> QHGKKDSKITDHFMRLPK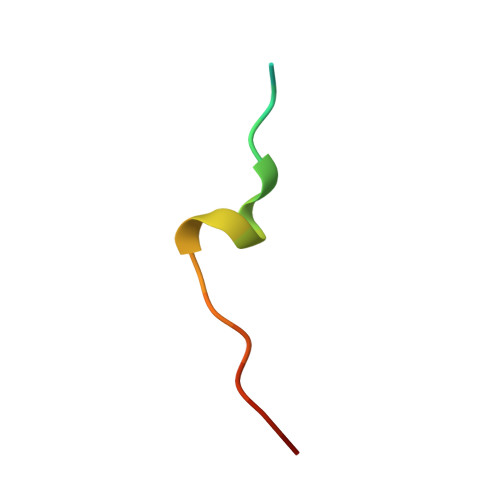A>AMLSPEALTTAVDAAQQAIALADTLDVLARVKTEHLGDRSPLALARQALAVLPKEQRAEAGKRVNAARNAAQRSYDERLATLRAERDAAVLVAEGIDVTLPSTRVPAGARHPIIMLAEHVADTFIAMGWELAEGPEVETEQFNFDALNFPADHPARGEQDTFYIAPEDSRQLLRTHTSPVQIRTLLARELPVYIISIGRTFRTDELDATHTPIFHQVEGLAVDRGLSMAHLRGTLDAFARAEFGPSARTRIRPHFFPFTEPSAEVDVWFANKIGGAAWVEWGGCGMVHPNVLRATGIDPDLYSGFAFGMGLERTLQFRNGIPDMRDMVEGDVRFSLPFGVGA[2x];>[2x]QSNAMRLPYSWLREVVAVGASGWDVTPGELEQTLLRIGHEVEEVIPLGPVDGPVTVGRVADIEELTGYKKPIRACAVDIGDRQYREIICGATNFAVGDLVVVALPGATLPGGFTISARKAYGRNSDGMICSAAELNLGADHSGILVLPPGAAEPGADGAGVLGLDDVVFHLAITPDRGYCMSVRGLARELACAYDLDFVDPASNSRVPPLPIEGPAWPLTVQPETGVRRFALRPVIGIDPAAVSPWWLQRRLLLCGIRATCPAVDVTNYVMLELGHPMHAHDRNRISGTLGVRFARSGETAVTLDGIERKLDTADVLIVDDAATAAIGGVMGAASTEVRADSTDVLLEAAIWDPAAVSRTQRRLHLPSEAARRYERTVDPAISVAALDRCARLLADIAGGEVSPTLTDWRGDPPCDDWSPPPIRMGVDVPDRIAGVAYPQGTTARRLAQIGAVVTHDGDTLTVTPPSWRPDLRQPADLVEEVLRLEGLEVIPSVLPPAPAGRGLTAGQQRRRTIGRSLALSGYVEILPTPFLPAGVFDLWGLEADDSRRMTTRVLNPLEADRPQLATTLLPALLEALVRNVSRGLVDVALFAIAQVVQPTEQTRGVGLIPVDRRPTDDEIAMLDASLPRQPQHVAAVLAGLREPRGPWGPGRPVEAADAFEAVRIIARASRVDVTLRPAQYLPWHPGRCAQVFVGESSVGHAGQLHPAVIERSGLPKGTCAVELNLDAIPCSAPLPAPRVSPYPAVFQDVSLVVAADIPAQAVADAVRAGAGDLLEDIALFDVFTGPQIGEHRKSLTFALRFRAPDRTLTEDDASAARDAAVQSAAERVGAVLRG

AaRSs catalyze the attachment of the correct amino acid to its cognate tRNA which then is used in protein synthesis on ribosomes. Phylogenetically phenylalanyl-tRNA synthetase (PheRS), belongs to the class II aaRSs, and it is a dimer of heterodimers (αβ)2, containing two α- (PheS) and two β- (PheT) subunits. Structural studies of PheRS have shown that the α subunit binds L-Phe and ATP and is responsible for esterification catalysis. At the same time, the β subunit is involved in the recognition of the cognate tRNA molecule and editing of mis-charged tRNA.

The protein-fragment interactions were analyzed using crystal structures for five of those fragments complexed with MtPheRS/tRNAPhe (DDD00107555 (D-555), DDD01008876 (D-876), DDD00805735 (D-735), DDD00079004 (D-004) and DDD00067116 (D-116)). All five fragments occupy the L-Phe site in the α subunit of the heterotetramer. The fragments’ orientation in these structures is very similar to the L-Phe substrate, however there are subtle differences in orientation and details of interactions. PIEDA showed that the phenyl ring or the bicyclic core of the fragments interact with residues αPhe255 and αPhe257 through hydrophobic interaction. One of two carbonyl groups of the D-555 interacts with αGln215 and αGly282 through hydrogen bonds. The core and the carbonyl oxygen of the oxazinone moiety interacts with αSer177 and αArg201 through hydrogen bonds, respectively. Fragment D-555 is unique in forming key interactions with αSer117, αPhe213 and αGly282 residues. However, the auxiliary pocket in the structures of PheRS with bound fragments was completely unoccupied offering an opportunity for fragment growth by adding hydrophobic substituents to explore the auxiliary pocket of MtPheRS.> METLVRPKPELLKLLKSVGA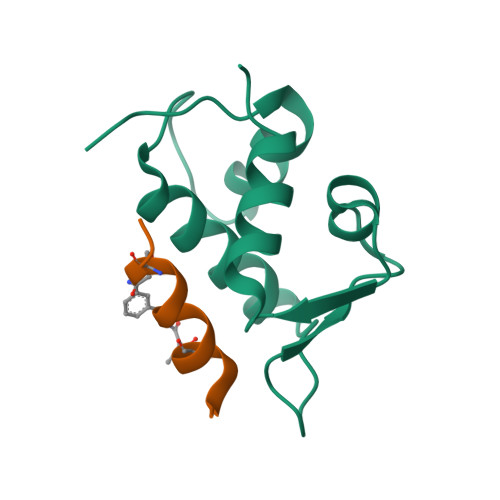QKDTYTMKEVLFYLGQYIMTKRLYDEKQQHIVYCSNDLLGDLFGVPSFSVKEHRKIYTMIYRNLVV;> LTFDQYWAQLDSAA>[5x]MNLTELKNTPVSELITLGENMGLENLARMRKQDIIFAILKQHAKSGEDIFGDGVLEILQDGFGFLRSADSSYLAGPDDIYVSPSQIRRFNLRTGDTISGKIRPPKEGERYFALLKVNEVNFDKPENARNKILFENLTPLHANSRLRMERGNGSTEDLTARVLDLASPIGRGQRGLIVAPPKAGKTMLLQNIAQSIAYNHPDCVLMVLLIDERPEEVTEMQRLVKGEVVASTFDEPASRHVQVAEMVIEKAKRLVEHKKD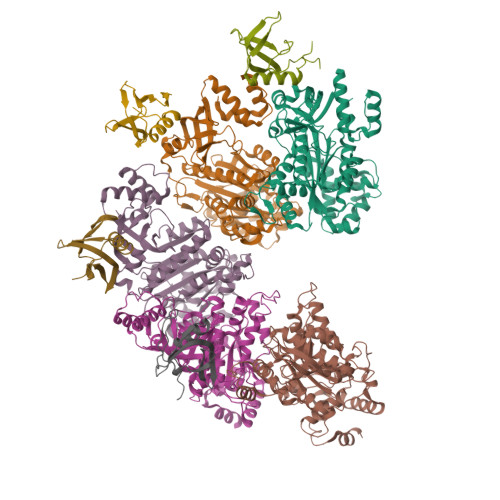VIILLDSITRLARAYNTVVPASGKVLTGGVDANALHRPKRFFGAARNVEEGGSLTIIATALIDTGSKMDEVIYEEFKGTGNMELHLSRKIAEKRVFPAIDYNRSGTRKEELLTTQEELQKMWILRKIIHPMGEIDAMEFLINKLAMTKTNDDFFEMMKRS;>[4x]AMGNDTYQPINCDDYDNLELACQHHLMLTLELKDGEKLQAKASDLVSRKNVEYLVVEAAGETRELRLDKITSFSHPEIGTVVVSES>MAGFWVGTAPLVAAGRRGRWPPQQLMLSAALRTLKHVLYYSRQCLMVSRNLGSVGYDPNEKTFDKILVANRGEIACRVIRTCKKMGIKTVAIHSDVDASSVHVKMADEAVCVGPAPTSKSYLNMDAIMEAIKKTRAQAVHPGYGFLSENKEFARCLAAEDVVFIGPDTHAIQAMGDKIESKLLAKKAEVNTIPGFDGVVKDAEEAVRIAREIGYPVMIKASAGGGGKGMRIAWDDEETRDGFRLSSQEAASSFGDDRLLIEKFIDNPRHIEIQVLGDKHGNALWLNERECSIQRRNQKVVEEAPSIFLDAETRRAMGEQAVALARAVKYSSAGTVEFLVDSKKNFYFLEMNTRLQVEHPVTECITGLDLVQEMIRVAKGYPLRHKQADIRINGWAVECRVYAEDPYKSFGLPSIGRLSQYQEPLHLPGVRVDSGIQPGSDISIYYDPMISKLITYGSDRTEALKRMADALDNYVIRGVTHNIALLREVIINSRFVKGDISTKFLSDVYPDGFKGHMLTKSEKNQLLAIASSLFVAFQLRAQHFQENSRMPVIKPDIANWELSVKLHDKVHTVVASNNGSVFSVEVDGSKLNVTSTWNLASPLLSVSVDGTQRTVQCLSREAGGNMSIQFLGTVYKVNILTRLAAELNKFMLEKVTEDTSSVLRSPMPGVVVAVSVKPGDAVAEGQEICVIEAMKMQNSMTAGKTGTVKSVHCQAGDTVGEGDLLVELE[6x];>[6x]MAAALRVAAVGARLSVLASGLRAAVRSLCSQATSVNERIENKRRTALLGGGQRRIDAQHKRGKLTARERISLLLDPGSFVESDMFVEHRCADFGMAADKNKFPGDSVVTGRGRINGRLVYVFSQDFTVFGGSLSGAHAQKICKIMDQAITVGAPVIGLNDSGGARIQEGVESLAGYADIFLRNVTASGVIPQISLIMGPCAGGAVYSPALTDFTFMVKDTSYLFITGPDVVKSVTNEDVTQEELGGAKTHTTMSGVAHRAFENDVDALCNLRDFFNYLPLSSQDPAPVRECHDPSDRLVPELDTIVPLESTKAYNMVDIIHSVVDEREFFEIMPNYAKNIIVGFARMNGRTVGIVGNQPKVASGCLDINSSVKGARFVRFCDAFNIPLITFVDVPGFLPGTAQEYGGIIRHGAKLLYAFAEATVPKVTVITRKAYGGAYDVMSSKHLCGDTNYAWPTAEIAVMGAKGAVEIIFKGHENVEAAQAEYIEKFANPFPAAVRGFVDDIIQPSSTRARICCDLDVLASKKVQRPWRKHANIPL

Propionyl-CoA carboxylase (PCC) and 3-methylcrotonyl-CoA carboxylase (MCC) are biotin-dependent carboxylases (BDCs) that catalyze the metabolism of odd-chain fatty acids, cholesterol, and specific amino acids. In contrast, PCC and MCC have their BC, CT, and BCCP domains divided into two chains: the α subunits contain the BC and BCCP domains, with an intermediate BC-CT interaction (BT) domain between them, while the β subunits solely consist of the CT domain. In humans, PCC and MCC catalyze the carboxylation of propionyl-CoA and 3-methylcrotonyl-CoA (MC-CoA), respectively. (**A, B**) The side view (left) and top view (right) of human PCC holoenzyme (PCC-apo) (**A**) and MCC holoenzyme (MCC-apo) (**B**). Both holoenzymes are dodecamers consisting of six α subunits and six β subunits.

We incubated the purified human BDCs with propionyl-CoA ([Fig figs1], D to G), which is the substrate of PCC, and determined the cryo-EM structures of the propionyl-CoA-bound PCC and MCC holoenzymes (referred to as PCC-PCO and MCC-PCO), at resolutions of 2.80 Å and 2.36 Å, respectively ([Fig figs2], [Fig figs3], E to H, [Fig figs4], E to H, [Fig figs6] and [Fig figs7], [Table tbls1] and [Fig figs2]). In each PCC holoenzyme, six propionyl-CoA molecules are observed binding to the six active sites of CT domains. Each binding site for propionyl-CoA is formed by the CT-C subdomain of one β subunit and the CT-N subdomain of another β subunit in the other layer ([Fig fig3]). The conformation of the propionyl-CoA binding pocket in the PCC-PCO structure is only slightly different from that in the PCC-apo structure ([Fig fig3]). The AMKM motif in the BCCP domain and the biotin covalently linked to it also show only minor conformational differences in the PCC-PCO structure compared to the PCC-apo structure ([Fig fig3]). The distances between the ureido ring carbonyl oxygen of the biotin and the main chain amide of the catalytic residues G437 and A438 in the corresponding CT domain in the PCC-PCO structure are more than 7 Å, which is too far for an efficient catalytic process ([Fig fig3]). This finding suggests that the biotin may need to relocate to a site that is closer to the catalytic residues to facilitate the carboxylation reaction. The binding mode of propionyl-CoA in our PCC-PCO structure is distinct from that in the ScPCC β subunit structure, but similar to that in the MePCC holoenzyme structure ([Fig fig3]). But the PCC-PCO structure shows that D440, which corresponds to D422 in the β subunit of ScPCC, is not directly involved in the interaction with propionyl-CoA or acetyl-CoA ([Fig fig3]).>[6x]PPGPPGPPGPPGPPGPP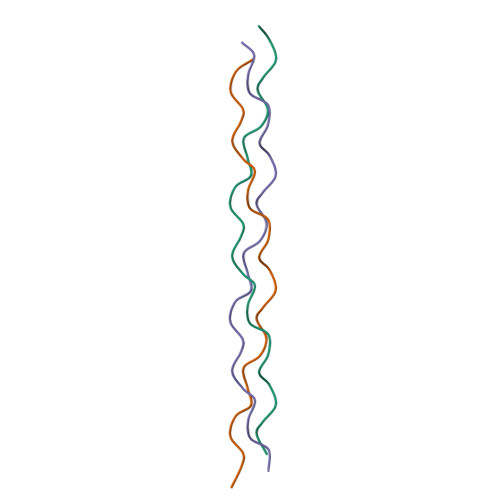GPPGPPGPPG> AETYEGD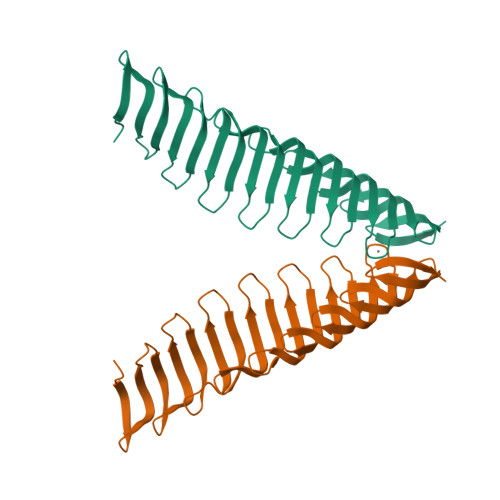WVDGKMQGRGTYFFADGGIYEGDWVDGKMEGKGVYKYLNGNKYEGEWINDMKNGYGTLAYVNGELYEGYWKNDKVHGKGTLTYSKGDKYIGEWKYAKKCGEGELIYASGDKFKGQWKNDKANGYGILLYNNGNKYEGEWLDDHRHGMGTFTCKEDGTIYSGHFQFNRKHGKGTLTFVNGHILQGIWNSGLLEKVINYELTPSSPWNDPDL Here we present the structural and functional studies of SCARB2, a functional receptor of the important human enterovirus 71 (EV71). SCARB2 is responsible for attachment as well as uncoating of EV71. SCARB2 is ubiquitously expressed and serves as a common receptor for all clinically isolated EV71 strains, CVA16, CVA7 and CVA14. SCARB2 (residues 37–430) consists of three domains arranged in a “Kidney” shape.

To gain an understanding of the molecular basis of SCARB2-mediated uncoating of EV71 under acidic conditions, we solved the crystal structures of the ectodomain of SCARB2 under both neutral (pH 7.5) (hereafter denoted as nSCARB2) and acidic conditions (pH 4.8) (hereafter denoted as aSCARB2). A striking difference in the position of the “cap” is observed between structures at acidic and neutral pH. The structure of aSCARB2 reveals a penetrable tunnel, which traverses the entire length of the molecule. In contrast, under acidic conditions, we propose that an alteration in the protonation state of H150 triggers the re-arrangement of the linker region connecting α4 with α5 such that the linker is now part of α5. Helix α4 is shortened in length, giving rise to a new linker (residues 146–150), that folds away from α7, connecting a much longer α5 with α4. More importantly, α5 moves towards α15 and together with the conformational change of W146, extends the lipid-transfer tunnel right through to the membrane-distal end of the molecule with an open entrance. This movement is facilitated by formation of new hydrogen bonds by R153 and E157. Additional electrostatic interactions between H150 and K161 of α5 and D394 and E397 of α15 further assist in the movement of α5. Under acidic conditions, such as encountered in the late endosome, parts of helices α4 and α5 of the viral binding domain of SCARB2 move away from helix α7, resulting in opening of the lipid-transfer tunnel. When exposed to acid pH in the late endo/lyso-somes, the cap undergoes conformational changes that lead to the opening of the lipid-transfer tunnel.

>[4x]IEKKIVLRNGTEAFDSWEKPPLPVYTQFYFFNVTNPEEILRGETPRVEEVGPYTYRELRNKANIQFGDNGTTISAVSNKAYVFERDQSVGDPKIDLIRTLNIPVLTVIEWSQVHFLREIIEAMLKAYQQKLFVTHTVDELLWGYKDEILSLIHVFRPDISPYFGLFYEKNGTNDGDYVFLTGEDSYLNFTKIVEWNGKTSLDWWITDKCNMINGTDGDSFHPLITKDEVLYVFPSDFCRSVYITFSDYESVQGLPAFRYKVPAEILANTSDNAGFCIPEGNCLGSGVLNVSICKNGAPIIMSFPHFYQADERFVSAIEGMHPNQEDHETFVDINPLTGIILKAAKRFQINIYVKKLDDFVETGDIRTMVFPVMYLNESVHIDKETASRLKSMI>MKGYTVPLSPRGIANLAPAPPWHYAGTVVGVEFFTDPAAAAATLPEGLTPDPDSAGRGVAMFIDWQYSSTGLEYLDPARSQYREFLITLDAHCNGAPVAWCPYIYVDNDAAMARGWVQGFPKKLGAVHQTRAYSVGGPGTPVLGPGGQFGATASSAGQRIAEAKITLEQPVPDPAALMSRPVINLRHFPRLAAGQHDQPAVHELVMSVLDDTAVSDAWVGTAD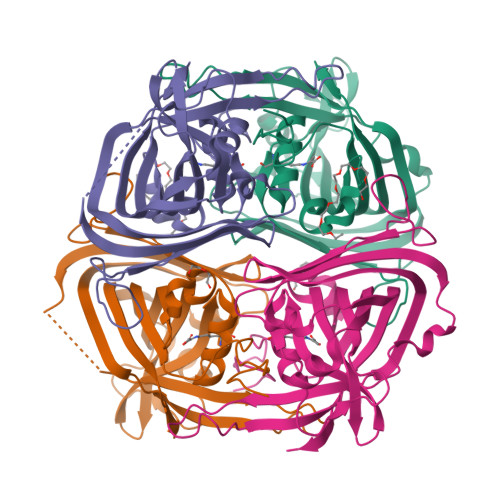LAFLPAHGEELADLPVRRTGKGFHFDLAYTVTDLMTLADHSA[4x]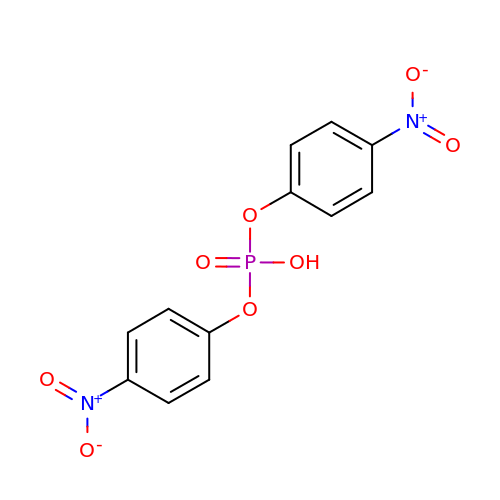bis(4-nitrophenyl) hydrogen phosphate | C12 H9 N2 O8 P | MHSVUSZEHNVFKW-UHFFFAOYSA-N> VQRVEGKLRASVEKGDYYEAHQMYRTLFFRYMSQSKHTEARELMYSGALLFFSHGQQNSAADLSMLVLESLEKAEVEVADELLENLAKVFSLMDPNSPERVTFVSRALKWS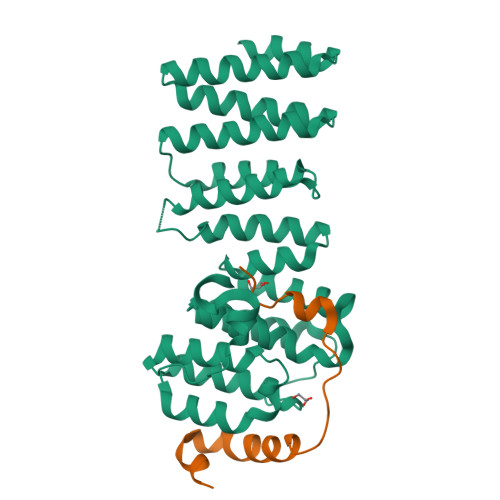SGGSGKLGHPRLHQLLALTLWKEQNYCESRYHFLHSADGEGCANMLVEYSTSRGFRSEVDMFVAQAVLQFLCLKNKSSASVVFTTYTQKHPSIEDGPPFVEPLLNFIWFLLLAVDGGKLTVFTVLCEQYQPSLRRDPMYNEYLDRIGQLFFGVPPKQTSSYGGLLGNLLTSL;> EPWAAAVPPEWVPIIQQDIQSQRKVKPQPPLSDAYLSGMPAKR>[18x]GSTGSSISTAVIDAINSGATLKDINAIPDDMMDDIYSYAYDFYNKGRIEEAEVFFRFLCIYDFY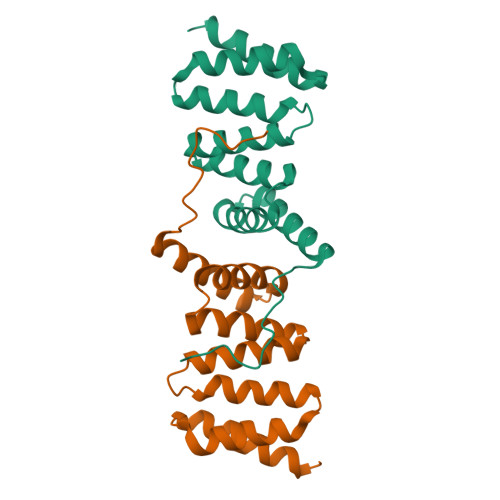NVDYIMGLAAIYQIKEQFQQAADLYAVAFALGKNDYTPVFHTGQCQLRLKAPLKAKECFELVIQHSNDEKLKIKAQSYLDAIQDIKE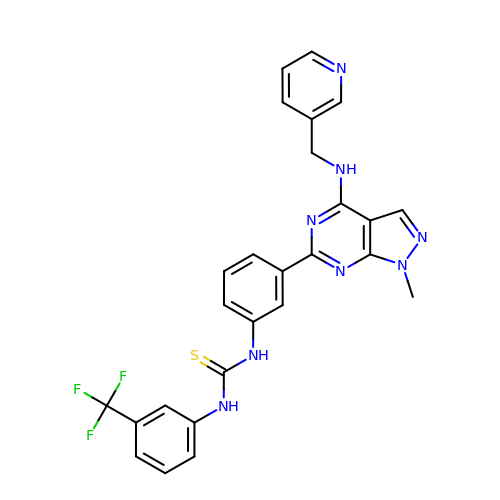1-[3-[1-methyl-4-(pyridin-3-ylmethylamino)pyrazolo[3,4-d]pyrimidin-6-yl]phenyl]-3-[3-(trifluoromethyl)phenyl]thiourea | C26 H21 F3 N8 S | UPEIYMKISINCQK-UHFFFAOYSA-N> LEAELHNCVVVQFDGPMSFYVQMESDVPALEQMTDKLLDAEQDLPAFSDLKEGALCVAQFPEDEVFYRAQIRKVLDDGKCEVHFIDFGNNAVTQQFRQLPEELAKPARYSRHCELDASTISKCDA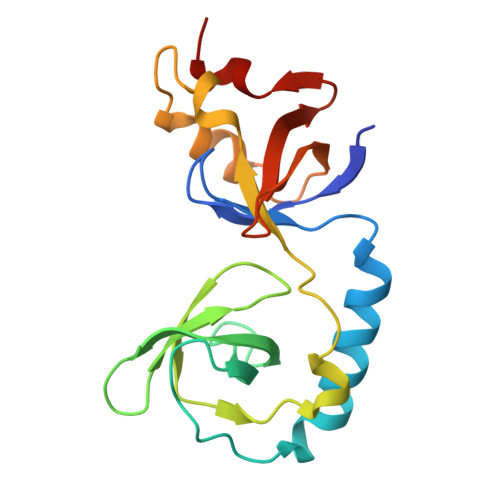ALLQSFIDTRFSETFQVEILATKGTGTHVVRLFYQSKNISEKLQECQ>[2x]MSDQLQMTDGMHIIVEALKQNNIDTIYGVVGIPVTDMARHAQAEGIRYIGFRHEQSAGYAAAASGFLTQKPGICLTVSAPGFLNGLTALANATVNGFPMIMISGSSDRAIVDLQQGDYEELDQMNAAKPYAKAAFRVNQPQDLGIALARAIRVSVSGRPGGVYLDLPANVLAATMEKDEALTTIVKVENPSPALLPCPKSVTSAISLLAKAERPLIILGKGAAYSQADEQLREFIESAQIPFLPMSMAKGILEDTHPLSAAAARSFALANADVVMLVGARLNWLLAHGKKGWAADTQFIQLDIEPQEIDSNRPIAVPVVGDIASSMQGMLAELKQNTFTTPLVWRDILNIHKQQNAQKMHEKLSTDTQPLNYFNALSAVRDVLREN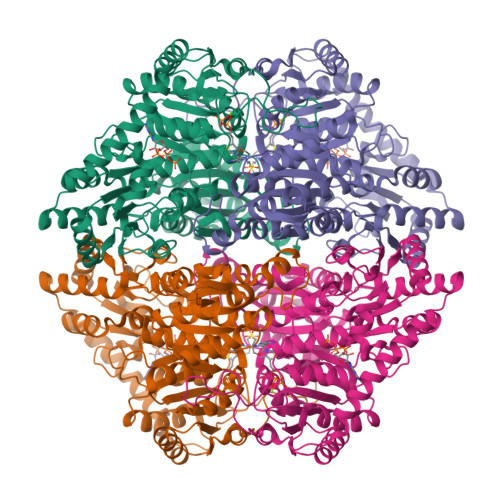QDIYLVNEGANTLDNARNIIDMYKPRRRLDCGTWGVMGIGMGYAIGASVTSGSPVVAIEGDSAFGFSGMEIETICRYNLPVTIVIFNNGGIYRGDGVDLSGAGAPSPTDLLHHARYDKLMDAFRGVGYNVTTTDELRHALTTGIQSRKPTIINVVIDPAAGTESGHITKLNPKQVAGN> MHHHHHHASGLVPRGSHMTRTTALKVLAGKKLTDLDPDEWAKAQASAERILVDVGTGDART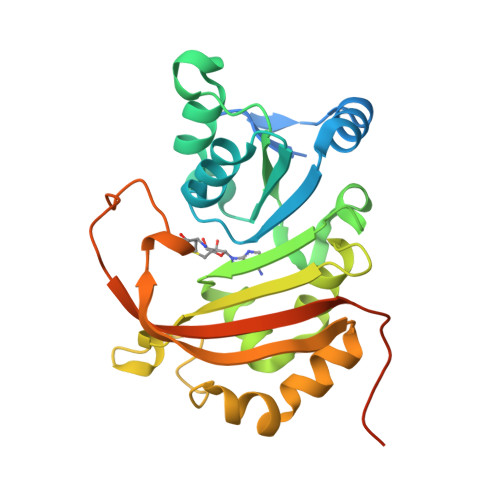AYRQAIAHPEWLVVGVDPAWQRMTETAVRAARKPAKGGAPNLVLVSSAIETVPAALHGVADEVMVLMPWGKLLRGVVLGEADVLSGLRAVAKPGAPLEISIGTSIWREPIPLEIRDLPELTPETVVSTGLTDRLAALGWQVADVRLVPHTDLDTISSSWARRLGSGATETVLHLRAVAVDPRDPVGTQHPAAESAQDTPEEPQRDV> QVVGWPP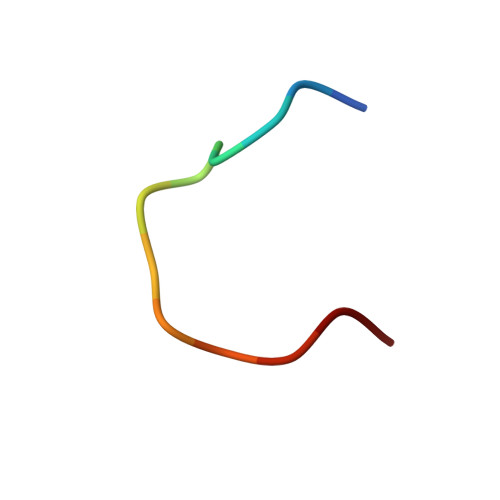VRNYRK> QEERSQQQDDIEELETKAVGMSNDGRFLKFDIEIGRGSFKTVYKGLDTETTVEVAWCELQDRKLTKSERQRFKEEAEMLKGLQHPN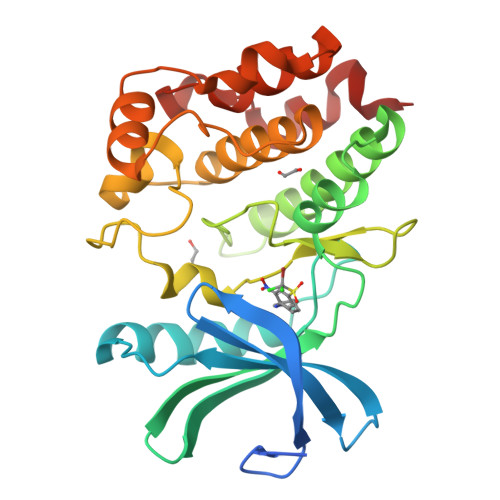IVRFYDSWESTVKGKKCIVLVTELMTSGTLKTYLKRFKVMKIKVLRSWCRQILKGLQFLHTRTPPIIHRDLKCDNIFITGPTGSVKIGDLGLATLKRASFAKAVIGTPEFMAPEMYEEKYDESVDVYAFGMCMLEMATSEYPYSECQNAAQIYRRVTSGVKPASFDKVAIPEVKEIIEGCIRQNKDERYSIKDLLNHAFFQEET> MASEAIKGAVVGIDLGTTNSCVAVMEGKQAKVLENAEGARTTPSVVAFTADGERLVGMPAKRQAVTNPNNTFYATKRLIGWRYDDPEVQKDIKNVPFKIVRASNGDAWVEAHGKLYSPSQIGAFVLMKMKETAENYLGHTAKNAVITVPAYFNDSQRQATKDAGQISGLNVLRVINEPTAAALAYGLDKSEDKVIAVYDLGGGTFDISILEIQKGVFEVKSTNGDTFLGGEDFDQALLRHIVKEFKRETGVDLTKDNMALQRVREAAEKAKCELSSSVQTDINLPYLTMDSSGPK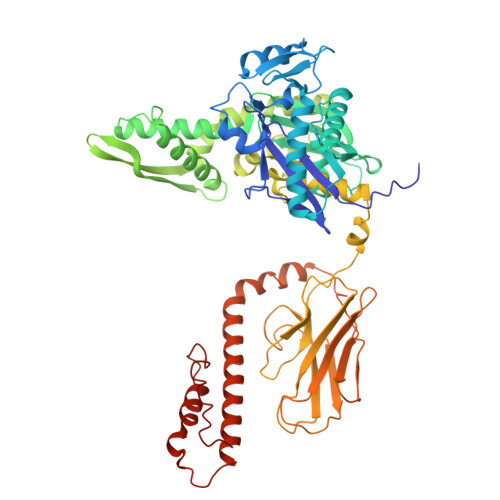HLNMKLTRAQFEGIVTDLIRRTIAPCQKAMQDAEVSKSDIGEVILVGGMTRMPKVQQTVQDLFGRAPSKAVNPDEAVAIGAAIQGGVLAGDVTDVLLLDVTPLSLGIETLGGVFTKLINRNTTIPTKKSQVFSTAADGQTQVEIKVCQGEREMAGDNKLLGQFTLIGIPPAPRGVPQIEVTFDIDANGIVHVSAKDKGTGREQQIVIQSSGGLSKDDIENMVKNAEKYAEEDRRKKERVEAVNMAEGIIHDTETKMEEFKDQLPADECNKLKEEISKMRELLARKDSETGENIRQAASS> MYNDDYIEEASFLNGSDVVILIDGVEELYMEEIKADFEQDEQSIKLLGCQNEISRVGTTKGSFS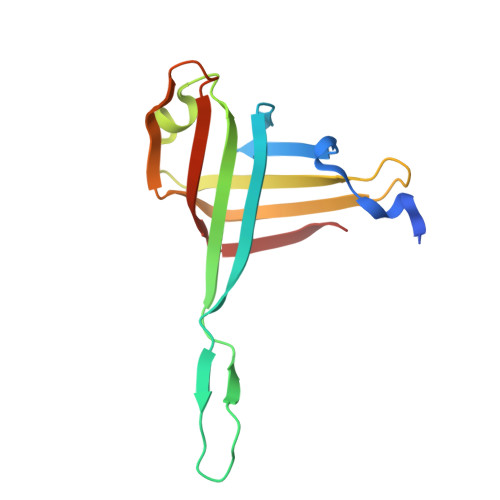LNGYKTDSKFAKLGFRSFEIIYNLSNSETLGYESIRLKNCRLKKLPLINSKAGEIVKIEVEGSFRGYDLLNEL> MISNSSAESISAPPNDSTIPHLAIDPFSLDFFDDPYPDQQTLRDAGPVVYLDKWNVYGVARYAEVHAVLNDPTTFCSSRGVGLSDFKKEKPWRPPSLILEADPPAHTRPRAVLSKVLSPATMKTIRDGFAAAADAKVDELLQRGCIDAIADLAEAYPLSVFPDAMGLKQEGREHLLPYAGLVFNAFGPPNELRQTAIERSAPHQAYVNEQCQRPNLAPGGFGACIHAFTDTGEITPDEAPLLVRSLLSAGLDTTVNGIGAA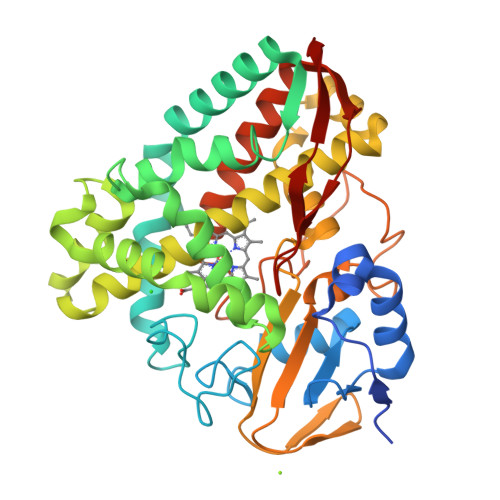VYCLARFPGELQRLRSDPTLARNAFEEAVRFESPVQTFFRTTTREVELGGAVIGEGEKVLMFLGSANRDPRRWSDPDLYDITRKTSGHVGFGSGVHMCVGQLVARLEGEVMLSALARKVAAIDIDGPVKRRFNNTLRGLESLPVKLTPA>[2x]MANTGEMKINWVSRYMPLLNKIAEEYSREKPLSGFTVGMSIHLEAKTAYLAITLSKLGAKVVITGSNPLSTQDDVAEALRSKGITVYARRTHDESIYRENLMKVLDERPDFIIDDGGDLTVISHTEREEV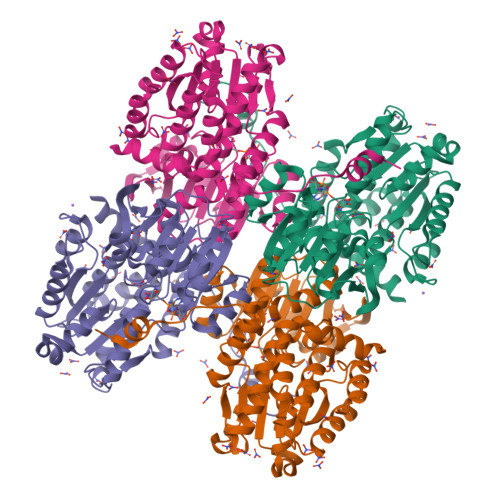LENLKGVSEETTTGVRRLKALEETGKLRVPVIAVNDSKMKYLFDNRYGTGQSTWDAIMRNTNLLVAGKNVVVAGYGWCGRGIALRAAGLGARVIVTEVDPVKAVEAIMDGFTVMPMKEAVKIADFVITASGNTDVLSKEDILSLKDGAVLANAGHFNVEIPVRVLEEIAVEKFEARPNVTGYTLENGKTVFLLAEGRLVNLAAGDGHPVEIMDLSFALQIFAVLYLLENHRKMSPKVYMLPDEIDERVARMKLDSLGVKIDELTEKQRRYLRSWQHHHHHH> SSDKGKLSLQDVAELIRARACQRVVVMVGAGISTPSGIPDFRSPGSGLYSNLQQYDLPYPEAIFELPFFFHNPKPFFTLAKELYPGNYKPNVTHYFLRLLHDKGLLLRLYTQNIDGLERVSGIPASKLVEAHGTFASATCTVCQRPFPGEDIRADVMADRVPRCPVCTGVVKPDIVFFGEPLPQRFLLHVVDFPMADLLLILGTSLEVEPFASLTEAVRSSVPRLLINRDLVGPLAWHPRSR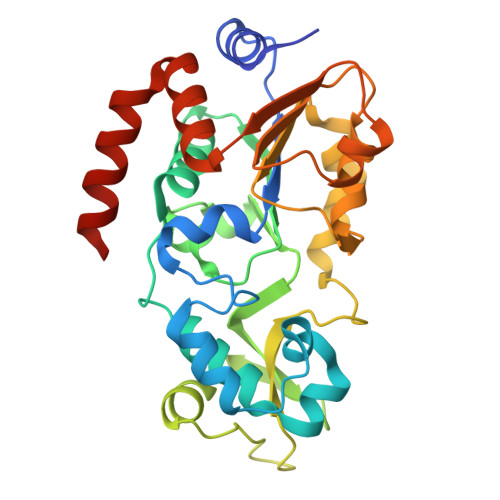DVAQLGDVVHGVESLVELLGWTEEMRDLVQRETGKLDGPDK>HHHHHHIEGRMKPSPEILALRWKDTCAHYSPHEWVAARNVVTANKAALADYFYECMLADPNAAFFLSDQLVKTKLHAAMQDWLESVYAAAPTEEYERTVAFQRKVGEVHARIDIPVHLVTRGACALIRRICELLDRDASLSAAQAAATCRYV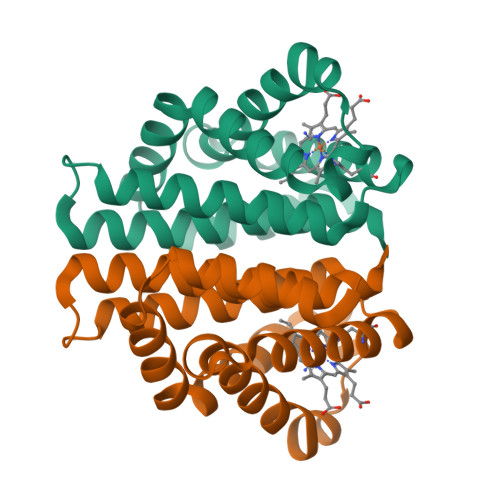ADVTMTAVEMMCHAYSVS[3x]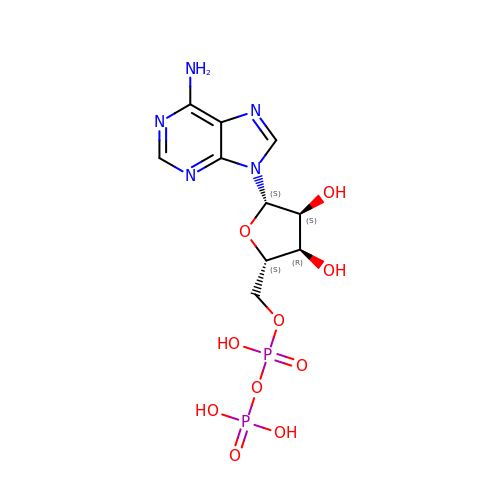L-ADENOSINE-5'-DIPHOSPHATE | C10 H15 N5 O10 P2 | XTWYTFMLZFPYCI-DEGSGYPDSA-N>MTTEQEFEKVELTADGGVIKTILKKGDEGEENIPKKGNEVTVHYVGKLESTGKVFDSSFDRNVPFKFHLEQGEVIKGWDICVSSMRKNEKCLVRIESMYGYGDEG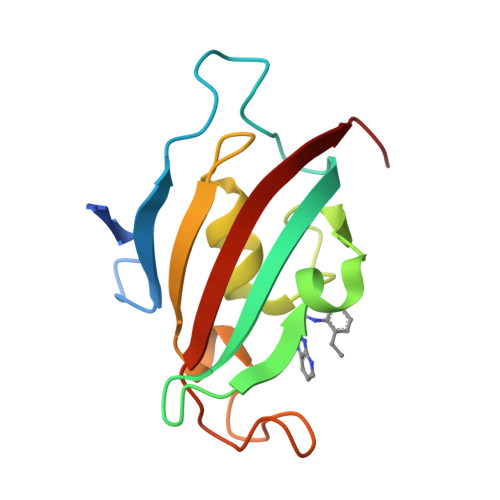CGESIPGNSVLLFEIELLSFRELE[3x]> SMSIHRRRTDPMVTLSSILESIINDMRDLPNTYPFHTPVNAKVVKDYYKIITRPMDLQTLRENVRKRLYPSREEFREHLELIVKNSATYNGPKHSLTQISQSMLDLCDEKLKEKEDKLARLEKAINPLLDDDDQVAFSFILDNIVTQKMMAVPDSWPFHHPVNKKFVPDYYKVIVNPMDLETIRKNISKHKYQSRESFLDDVNLILANSVKYNGPESQYTKTAQEIVNVCYQTLTEYDEHLTQLEKDICTAKEAALEEAELESLD

Bromodomains (BRDs) are protein interaction modules that specifically recognize ε-N-lysine acetylation motifs, a key event in the reading process of epigenetic marks. The 61 BRDs in the human genome cluster into eight families based on structure/sequence similarity. Despite large sequence variations, all BRD modules share a conserved fold that comprises a left-handed bundle of four α helices (αZ, αA, αB, αC), linked by loop regions of variable length (ZA and BC loops), which line the Kac binding site and determine binding specificity. The four helices form a deep cavity that is extended by the two loop regions (ZA and BC loops), creating a largely hydrophobic Kac binding pocket.

Multiple protein interaction modules can be tightly linked to form a single stable interaction domain, or they can be connected by flexible linker sequences allowing conformational adaptation to diverse sequences motifs. In contrast, the two BRDs in TAF1 are free to orient independently as shown by the different domain orientations in the dual-domain structure determined here and a previously published model (Jacobson et al., 2000). The frequent combination of multiple interaction modules in the same protein suggests that the epigenetic reading process involves concomitant recognition of several PTMs. Insertions x6 are present in the C-terminal BRDs of TAF1 and TAF1L and possibly PRKCBP1.>MKSNEHDDCQVTNPSTGHLFDLSSLSGRAGFTAAYSEKGLVYMSICGENENCPPGVGACFGQTRISVGKANKRLRYVDQVLQLVYKDGSPCPSKSGLSYKSVISFVCRPEAGPTNRPMLIS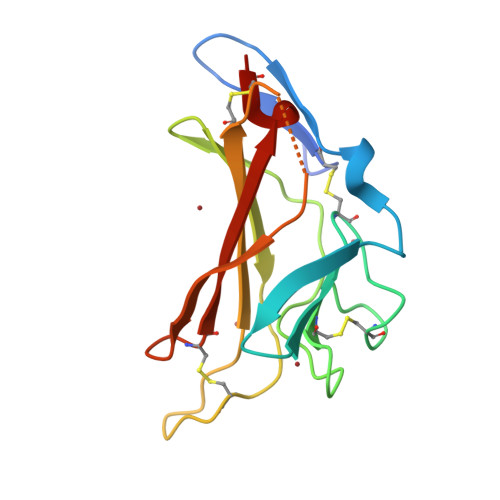LDKQTCTLFFSWHTPLACEQAT[2x]>ATQGVFTLPANTQFGVTAFANSAGTQTVNVQVNNETVATFTGQSTNNAIIGSKVLNSGGGGKVQILVSVNGRSSDLVSAQVILANELNFALVGSEDSTDNDYNDAVVVINWPLG[4x]

Two extracellular carbohydrate-binding proteins, LecA (PA-IL) and LecB (PA-IIL), are virulence factors and necessary for adhesion and biofilm formation. LecA binds to d-galactose; LecB from the strain PAO1 shows high binding affinities for l-fucose and reduced binding to d-mannose and their glycoconjugates. The genes of both P. aeruginosa lectins lecA and lecB are part of the core genome25 and while LecA is highly conserved, LecB shows sequence variation in 15 amino acids in PA14 compared to PAO1. Despite high sequence variations, biophysical characterization uncovered that both variants possess very similar glycan binding preferences, although very surprisingly LecBPA14 generally displays 2- to 7-fold higher affinities.

LecBPA14 was cloned, recombinantly expressed and purified from E. coli. In analogy to LecBPAO1,41 the 1.70 Å resolution native structure of LecBPA14 shows the lectin as homotetramer with the four carbohydrate recognition domains (CRD) containing two Ca2+-ions each located on the vertices of a pseudotetrahedron. A direct binding of G114 to one Ca2+-ion from the neighboring monomer stabilizes the tetrameric structure of the lectin, which was confirmed in solution by dynamic light scattering experiments (Fig. S4†). Notably, the structural alignment of LecBPA14 and LecBPAO1 revealed that all amino acid variations in LecBPA14 are located exclusively on the outer surface of the tetramer. Mutations at the interfaces of the tetramer subunits are not present, and thus the oligomerization of LecB is conserved. The crystal structure of LecBPA14 and comparison to its PAO1 homolog revealed the localization of all mutated amino acids on the outer surface of the LecB tetramer some of which are located in or near the carbohydrate binding site.> MSLQGIHLSDLSYKHAILKESQYTIKRDVGTTTAVTPSSLQQEITLLCGEILYAKHADYKYAAEIGIQYISTALGSERVQQILRNSGSEVQVVLT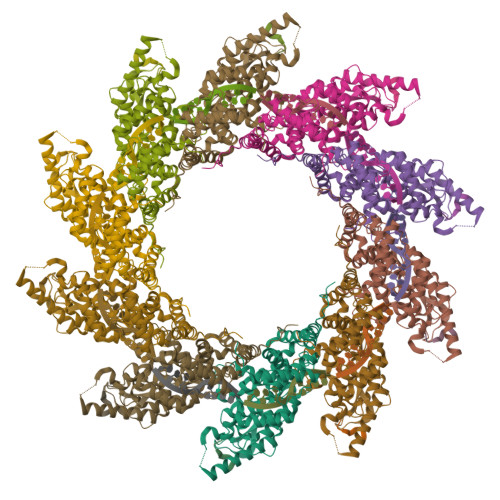RTYSLGKIKNNKGEDLQMLDIHGVEKSWVEEIDKEARKTMATLLKESSGNIPQNQRPSAPDTPIILLCVGALIFTKLASTIEVGLETTVRRANRVLSDALKRYPRMDIPKIARSFYDLFEQKVYHRSLFIEYGKALGSSSTGSKAESLFVNIFMQAYGAGQTMLRWGVIARSSNNIMLGHVSVQAELKQVTEVYDLVREMGPESGLLHLRQSPKAGLLSLANCPNFASVVLGNASGLGIIGMYRGRVPNTELFSAAESYAKSLKESNKINFSSLGLTDEEKEAAEHFLNVSDDSQNDYE;> DIYQLIM> ATLSSKPIIKGENLAYSMDEKVDLMKGITATDIEDGNITSKVQIKSSDFVEGKSGIFTVVYSVTDSDGLTSECSRTIAVTDKETQLSDLNWKSATIGSGSVRKD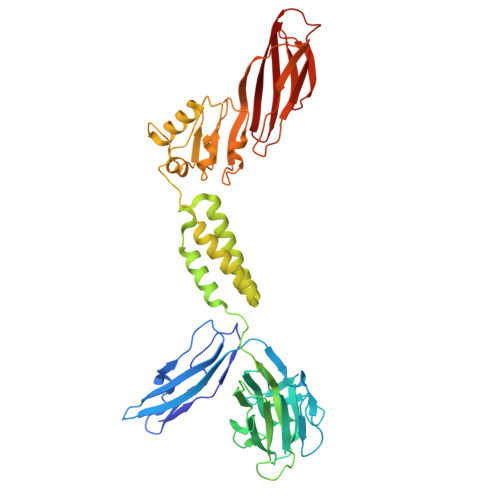RAVSGNQIRLLNEDNSVETFAKGIGTHSYSEIVYNSEGYDIFDTWVGIDRHVADKKVSSVKFKVYVDGELKAETDVMRIDTPKKRLVVDVRNSKEIKLVVDVADNGNNWDHADWADAKFRNLAEYDASELNKAIEEAKKLDLNNYTEESSEALKNAISKGEEALLSKDKETINSALEELNKEMNSLVKVDLNAVINIPDKYLLKSIQNQLNKTGDITLGDMYSLTTLTLSGVEDLTGLENAKNLETLNMDYNEVKDLRPLSKLKKLNTLNAQEQFIAAGELKPSNGKVIGDSKVYNREGKNVAKTIRVVDKNGNTILEQDAKDEFTINTKDLSSGLYGVHVLFEDEGFSGVMFYLFNV> MKQNINIGNVVDDGTGDYLRKGGIKINENFDELYYEL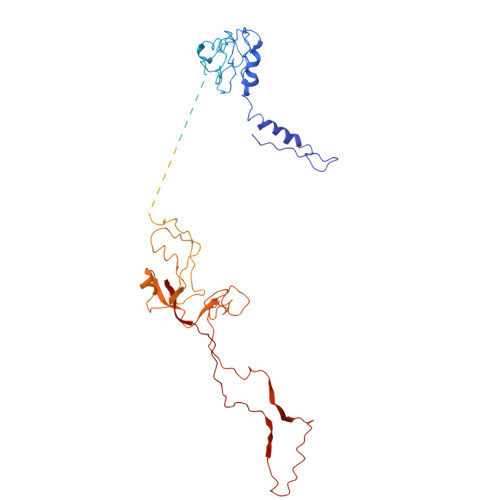GDGDVPYSAGAWKTYNASSGQTLTAEWGKSYAINTSSGRVTINLPKGTVNDYNKVIRARDVFATWNVNPVTLVAASGDTIKGSAVPVEINVRFSDLELVYCAPGRWEYVKNKQIDKITSSDISNVARKEFLVEVQGQTDFLDVFRGTSYNVNNIRVKHRGNELYYGDVFSENSDFGSPGENEGELVPLDGFNIRLRQPCNIGDTVQIETFMDGVSQWRSSYTRRQIRLLDSKLTSKTSLEGSIYVTDLSTMKSIPFSAFGLIPGEPINPNSLEVRFNGILQELAGTVGMPLFHCVGADSDDEVECSVLGGTWEQSHTDYSVETDENGIPEILHFDSVFEHGDIINITWFNNDLGTLLTKDEIIDETDNLYVSQGPGVDISGDVNLTDFDKIGWPNVEAVQSYQRAFNAVSNIFDTIYPIGTIYENAVNPNNPVTYMGFGSWKLFGQGKVLVGWNEDISDPNFALNNNDLDSGGNPSHTAGGTGGSTSVTLENANLPATETDEEVLIVDENGSVIVGGCQYDPDESGPIYTKYREAKASTNSTHTPPTSITNIQPYITVYRWIRIA5-methyl-6-{[3-(trifluoromethoxy)phenyl]sulfanyl}thieno[2,3-d]pyrimidine-2,4-diamine | C14 H11 F3 N4 O S2 | 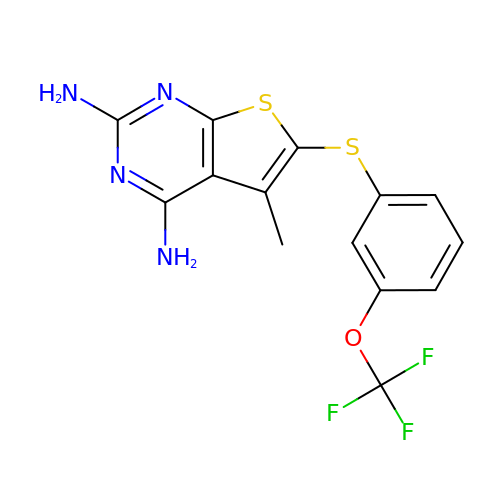DAABFILHHVUIKM-UHFFFAOYSA-N> MDSIDEQIA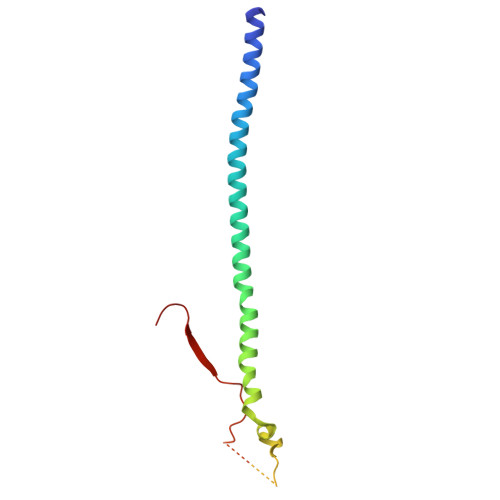IKRKELQSLQKITSLTDGLKIQLTELNEQIKEMGMNADSVAQLMNNWDSIINNISQASLGLLQYAEGDYEIGPWKDSKKKESEQSNETGLEAQENDKNDEDNDEDEDLVPLPETMVRIRVDGNE> PPTLQRCCRQLRNVSPFCRCPSLRQAVQSAQQ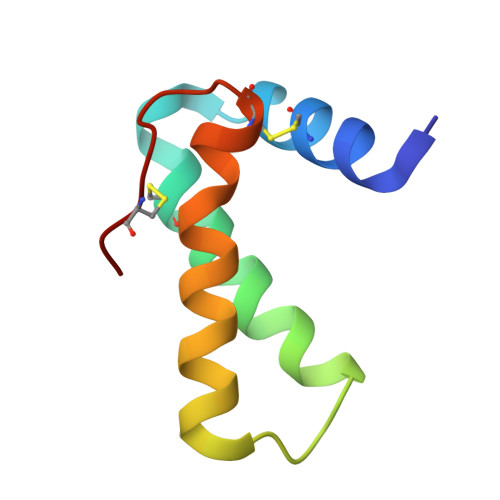QQGQVGPQQVGHMYRVASRIPAICNLQPMRCPF>[4x]GGSEQEIVNLFIPTQAVGAIIGKKGAHIKQLARFAGASIKIAPAEGPDVSERMVIITGPPEAQFKAQGRIFGKLKEENFFNPKEEVKLEAHIRVPSSTAGRVIGKGGKTVNELQNLTSAEVIVPRDQTPDENEEVIVRIIGHFFASQTAQRKIREIVQQVKQQEQK

In mammals, there are three IMP family members (ZBP1, IMP2, and IMP3). Each protein contains six canonical RNA-binding domains, two RNA recognition motif (RRM) domains and four hnRNP K homology (KH) domains. These RNA-binding domains are arranged into three pairs (RRM12, KH12, and KH34). In vivo functional studies as well as in vitro work suggested that KH34 domains are responsible for RNA recognition.

Similar to ZBP1KH34, we found that the individual KH3 and KH4 domains of IMP2 adopted the type 1 KH fold (βααββα) and were also arranged in an anti-parallel pseudo-dimer orientation. The overall structures of IMP2KH34 and ZBP1KH34 are almost identical (RMSD of 0.5 Å for all Cα atoms). We observed that IMP2KH34 had lower affinity to the ß-actin C28 zipcode RNA (Kd = 161 nM) compared with ZBP1KH34 (Kd = 15 nM). From the last round of selection, we identified a bipartite RNA element that included a 5′ CA element, CU-CA-C, followed by ten nucleotides and then a variable 3′ GG element, (A/U)-GG-(A/U). We found that the 5′ CA and the 3′ GG RNA element were bound specifically by the KH3 and KH4 protein domain, respectively. We hypothesized that the highly conserved GXXG motifs mediate phosphate backbone interactions and that the variable loops functioned to recognize specific nucleobases. To determine if the variable loops mediate differences in RNA-binding between ZBP1KH34 and IMP2KH34 we generated a chimeric protein where amino acids present near both variable loops of IMP2KH34 were exchanged with the corresponding amino acids present in the same position on ZBP1KH34 variable loops. We found that this exchange converted IMP2 into a ZBP1 like binding protein, which bound to the ß-actin zipcode, the ZBP1 RNA-binding element. We observed that only four amino acid mutations in the KH3 domain were necessary to allow IMP2 to bind to the ß-actin zipcode with nearly equal affinity to ZBP1KH34.> KETAA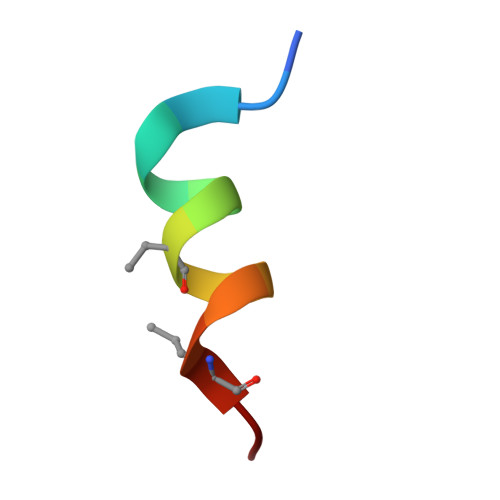AKAERQHLDS QUINACRINE MUSTARD | C23 H28 Cl3 N3 O | 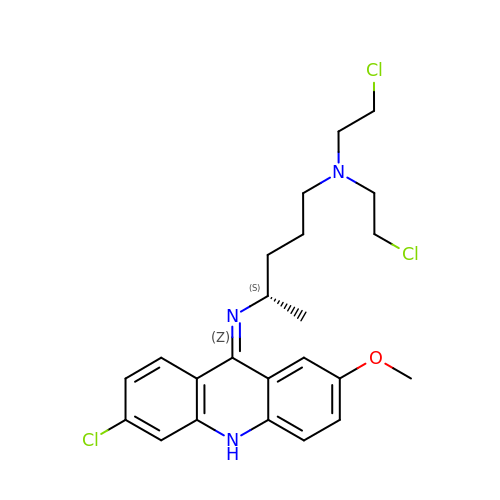UKOBAUFLOGFCMV-INIZCTEOSA-N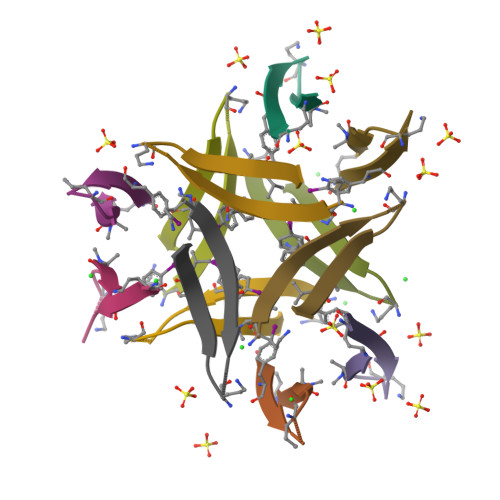>AYLLFYTEAKVAAAVK[6x];>AYLLFYTEAKVALAVK[6x]>[2x]MRDLYRNTNTFMIRTPIFSIDNYYEFFRKDGESDKIKDRLLEICNNSVFREAILVSSKSLYSTIIDFCDGKEIKKFDYFLQSIYKYLIRMSMRPTPFGLFSGVDFGKYAEETVISYENDNFKKFARPDLEWIIKIVKELEDNHYKNLTFKINDSIFIKGERALLIHSTDKEDNNRIGEISIRATKPFMRTYDLAKDGIEYNKLKYILIDEYSIEDESKIDNFLKQLIEREFLISNLRPPLTVLDQFDYLINEVKKAEIEIPLVDELTEIKEKLKLYNETPVGAGEETYLELYKKMESVANVKNILQVDMKLNLRDKKINKKIISDVNDLMNILLDLSMSIENPEPFLSKYKQEFIEKYGQDREISLLEMLDNDIGIGPPMNYERPRNNRSLDVSVNELLDNNVRDYFMEKYFQALKTNSRNIAIRDDEIKNLELQKIDYENIPDSLEINLLVKNKSEDNLSDEFQYYIGPNLGSTSAGKSFGRFSHMMSEPKKFFEELDERNIELIDSEEYVTCEISYLPSEVRNANVTRNIHSSEYEMSLFTNGSKDNLYRIKLNDIYIGLENNTFYAKSKTLNKKLLLTINNMLNPQTAPNAIRFLNDISLDEKKLWYKFVWSDVYKDFSYIPAIKYKNFVIMPETWKMNKINMKINKKTEFNEFKNQFNDYRIKYGVPQYVYITFADNRILLNLDDEQCVKILYHECKNSFNEIILNSYEEEGVNIVKESHKDYICELVIPLTKIKQETISDKVSARMLSSDISSLSKERVKDPFDEWLYIKLYGISSNVDDLIAYYISEFCNELVEEEIISKYFFMRYVDPEQHIRLRLNSSQEKLLMIYPKIREWLSMIRKKGLMTYFSIDSYDREIERYGGIELINIAEKVFFFDSIVTEDILRAKREGSFDFCDEIIGMISVVHYMESFGLPYAKQVEFLRSQVSSSEYREDFKQKRTEYMKLCNSNKDWEGLRESEEGNILIEILNKRRKIIEYYGNKVRENEEVSTDLSILDSIIHLNCNRMFGIDREFEKKVRALASHALYALKHFKS;>[2x]MGKLDDFDLDVKVKADTTKVGPAITSKSLCTPGCITGVLMCITQNSCVSCKSCIKC

Maddinglicin A (MadA) produced by Clostridum maddingley belongs to a group of antimicrobial peptides, the so-called lantibiotics or in brief LanA1. The first necessary step is the dehydration of serine and threonine residues, which is catalyzed by the MadB enzyme in the case of MadA. The structure of MadB in the apo-state was determined at an overall resolution of 2.7 Å. MadB is composed of an N-terminal glutamylation (residues 1–741) and a C-terminal elimination (residues 742–1038) domain (see Fig. S1 for the sequence). MadB forms a homodimer as already demonstrated by SEC-MALS with a bifurcate cleft-like structure in the center.

To elucidate conformational changes upon substrate binding, we also determined the structure of MadB in complex with the MadA variant MadL3 at an overall resolution of 3.1 Å. MadL3 compromises the LP of MadA including the first ten N-terminal amino acids of the CP. Electron density for the stretch of residues −20LDDFDLDVKVKA−9 was clearly resolved and could be built. The LP of MadA binds to the RRE element in MadB, which is present in the majority of prokaryotic RiPP classes. Substrate binding induced the formation of a four-stranded, anti-parallel β-sheet, which is a three-stranded, anti-parallel β-sheet in the apo-state. We investigated the interactions of MadB to its substrate via LigPlot+27 with standard settings, which mostly found backbone to backbone or residue to backbone hydrogen interactions (MadB-MadA: Thr184 – Asp−18; Gln225 – Leu−15; Arg182 – Asp−19 and Asp−16 ; Arg161 – Asp−14; Ser180 – Lys−12 ; Gly177 – Lys−10), but also some side chain to side chain interactions were observed (MadB-MadA: Lys218 – Asp−19; Glu178 – Lys−10; Asp785 – Lys−12). Beside hydrogen bond interactions also hydrophobic interactions could be observed for the amino acids F−17, L−15, V−13, V−11 of the MadA LP with the RRE of MadB (I176, I179, I181, P186, F187, I213, I219, F222). Interestingly, most interactions originate from amino acids of the GD, but also interactions from the ED of the opposing monomer towards the substrate were observed (e.g., Asp785). Residues 164–179 rotated by 8°, which is a prerequisite for substrate binding and formation of the RRE as the β-strand of the LP would severely clash with the loop in its position in the apo structure and thereby prevent binding of the LP as it acts as a lid closing the pathway for the substrate to bind. In the case of the ligand-bound state, hydrophobic interactions are formed with Ser154, Ile155, Arg229, Tyr518, Phe542, Leu519, Pro592, and Ile595 as well as Val−5, Lys−6, Val−7 and Ala−9 of the LP.> MRGSHHHHHHGMASLVPRGSVLPQLSPEQLGMI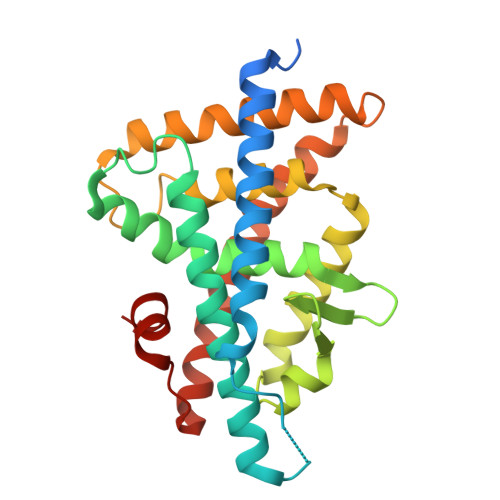EKLVAAQQQCNRRSFSDRLRVTPWPIAPDPQSREARQQRFAHFTELAIVSVQEIVDFAKQLPGFLQLSREDQIALLKTSAIEVMLLETSRRYNPGSESITFLKDFSYNREDFAKAGLQVEFINPIFEFSRAMNELQLNDAEFALLIAISIFSADRPNVQDQLQVERLQHTYVEALHAYVSINHPHDPLMFPRMLMKLVSLRTLSSVHSEQVFALRLQDKKLPPLLSEIWDVHE> MDTSTTASV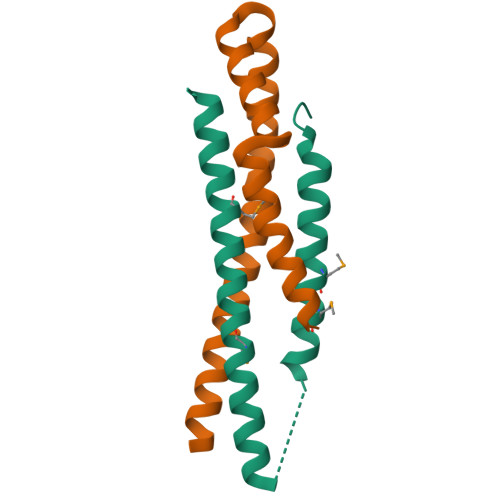ASANASTSTSMAYDLGSMSKDDVIDLFNKLGVFQAAILMFAYMYQAQSDLSIAKFADMNEASKESTTAQKMANLVDAKIADVQSSSDKNAKAQLPDEVISYINDPRNDITISGIDNINAQLGAGDLQTVKAAISAKANNLTTTVNNSQLEIQQMSNTLNLLTSARSDMQSLQYRTISGISLGK;> MGIVSQTRNKELLDKKIRSEIEAIKKIIAEFDVVKESVNELSEKAKTDPQAAEKLNKLIEGYTYGEERKLYDSALSKIEKLIETLSPARSKSQST> MAHHHHHHMLVEQRTYWLKPGSVSTFLSLYEAEGLAIQAGALGRLLGYYFSETGDLNRVIQLWG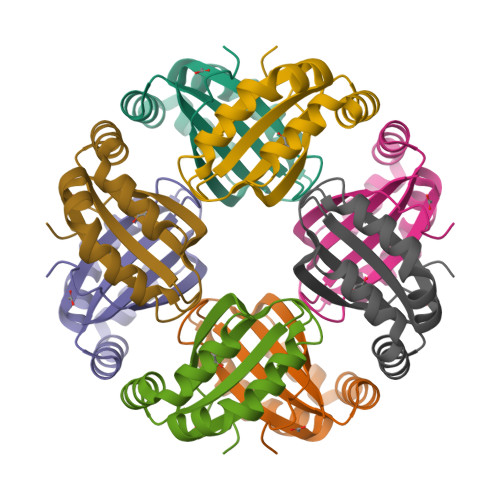FDSFEDRTRRKAILSGNPQWKSFVGRAGSMIERQSTELLTPAPFSPVS>SNATAQQWNKDVVGWNLGNEFECSAPGQDGESMQIGNPDGSIHAETAWGNPVVTKKMIQAVKKAGFNAIRIPIRWQCHITNAQAMSIDKAWIARIKEVVGWCLDNGLKVIINVHHEKWLESRPTYQYKEENCQKLALLWMNIASEFANYDSRLAFAGTNEVHIRDNWGKPTAENLEVQNAYNQIFVDVVRATGGNNAKRHLILQTYVCNPWFGIENGDFIIPKDAEGNGNNYMSVEFHYYQPWSYAGDCTYDYWGDAYKDAGKIPADNEKTMTDFFDKAVNTWSNKGLGIVIGEWGV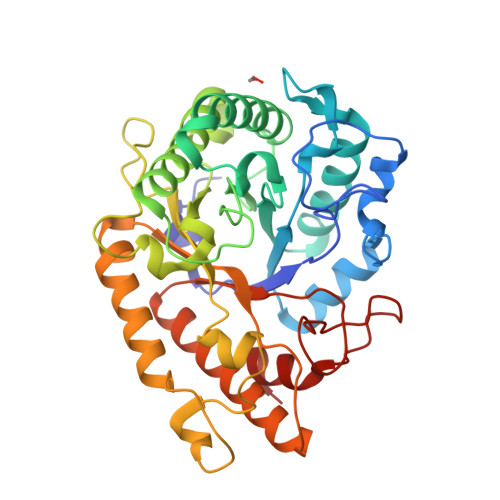TDHYKSNSEKVHENMTYYCKFLTTEARKRGFSTFVWDNNHFGNGSEKYGIFDRFKSMKVNAPWILEGIFGK[4x]>[6x]MASITDKDHQKVILVGDGAVGSSYAYAMVLQGIAQEIGIVDIFKDK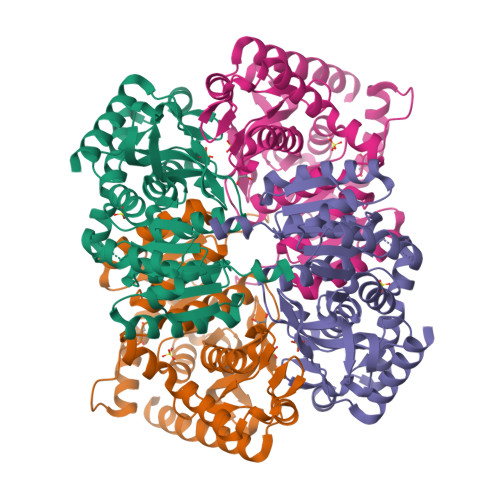TKGDAIDLEDALPFTSPKKIYSAEYSDAKDADLVVITAGAPQKPGETRLDLVNKNLKILKSIVDPIVDSGFNGIFLVAANPVDILTYATWKLSGFPKNRVVGSGTSLDTARFRQSIAKMVNVDARSVHAYIMGEHGDTEFPVWSHANIGGVTIAEWVKAHPEIKEDKLVKMFEDVRNKAYEIIKLKGATFYGIATALARISKAILNDENAVLPLSVYMDGQYGLNDIYIGTPAVINRNGIQNILEIPLTDHEEESMQKSASQLKKVLTDAFAKNDIETRQ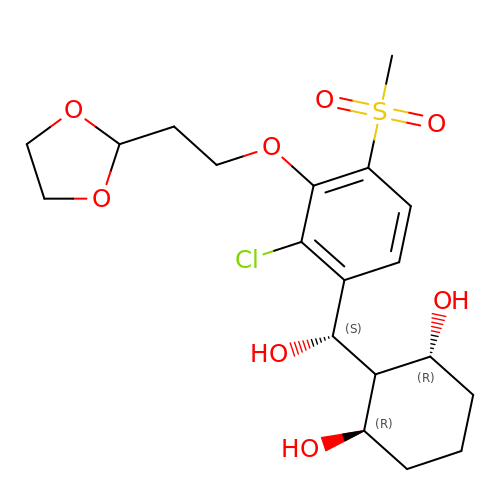(1R,3R)-2-[(S)-[2-chloranyl-3-[2-(1,3-dioxolan-2-yl)ethoxy]-4-methylsulfonyl-phenyl]-oxidanyl-methyl]cyclohexane-1,3-diol | C19 H27 Cl O8 S | HSPYNMFOCRTYFY-SNUQEOBHSA-N>NGSEWSYTNILTGPETWHEHYKNMCSGYYQSPIDLKTDISTLDLKLKTVIIYRNTSSTETTTIQNNGHSAEVKFPRNTWFISFDGILDYKYEIIQMHFHWGNTDDRGSEHTIDGFRFPLEGHIVSFRRQMYSSPSEAIGRPGGLAVLGIMHQIVESIKYEQTAFKAYNNFSGVLNSQFVPPNNSTIDDINLALLLSLLNPSRYFRYLGSLTTPPCTENVLWTVFIDPVLITREQINLFRNLPYGSNEKQTRMGDNFRPIQLLNPIDTLASRTLYRATARG[2x]

Carbonic anhydrases (EC 4.2.1.1) are widespread metallo­enzymes that can be clustered into eight families according to their amino-acid characteristics and differences in their active centers. They are present in all living organisms, catalyzing the hydration of carbon dioxide to bicarbonate and a proton. Clorsulon is an anthelmintic drug that is clinically used against Fasciola hepatica. For this purpose, the inhibitory activity and isoform selectivity of clorsulon was studied using human CA I and S. mansoni CA, revealing different modes of binding of clorsulon that explain its inhibitory potency against the two enzymes.

On the other hand, SmCA from S. mansoni was strongly affected by clorsulon (K i = 224.7 nM) and AAZ (K i = 42.5 nM), despite the latter being more potent. The benzenesulfonamide scaffold showed the same binding mode with the hydrogen bond between the O atom of the sulfonamide group and Thr231 stabilizing the binding of the inhibitor, as in the case of the complex with hCA I. In addition, this moiety formed a water bridge to Thr232. The second sulfonamide moiety played an important role in the location of the inhibitor; indeed, three hydrogen bonds were observed to Thr232, Tyr27 and Asn86, blocking the scaffold in a hydrophilic pocket inside the active site. Indeed, His200 in hCA I reduces the space available for the clorsulon tail and forces the second sulfonamide moiety (which is bulkier than the amino group) to move towards Gln92 (Gln115 in SmCA). On the other hand, in SmCA this residue is replaced by Thr232 with a less bulky side chain, which makes the active site more accessible, driving the sulfonamide moiety towards a more hydrophilic pocket, with a rotation of 130° with respect to the hCA I complex, and also allowing the formation of interactions with Tyr27 and Asn86 (Tyr7 and Val62 in hCA I). Taken together, these observations could explain the different inhibition potencies of clorsulon against hCA I and SmCA and the 20-fold selectivity for SmCA over hCA I.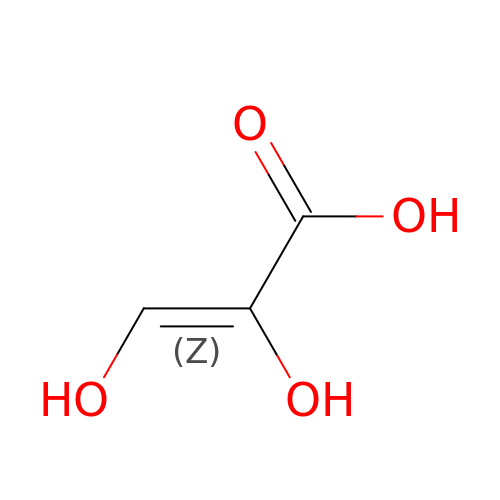(Z)-2,3-bis(oxidanyl)prop-2-enoic acid | C3 H4 O4 | XHDBNNIXWWTOFN-UPHRSURJSA-N> MPKLVTWMNNQRVGELTKLANGAHTFKYAPEWLASRYARPLSLSLPLQRGNITSDAVFNFFDNLLPDSPIVRDRIVKRYHAKSRQPFDLLSEIGRDSVGAVTLIPEDETVTHPIMAWEKLTEARLEEVLTAYKADIPLGMIREENDFRISVAGAQEKTALLRIGNDWCIPKGITPTTHIIKLPIGEIRQPNATLDLSQSVDNEYYCLLLAKELGLNVPDAEIIKAGNVRALAVERFDRRWNARRTVLLRLPQEDMCQTFGLPSSVKYESDGGPGIARIMAFLMGSSEALKDRYDFMKFQVFQWLIGATQGHAKNFSVFIQAGGSYRLTPFYDIISAFPVLGGTGIHISDLKLAMGLNASKGKKTAIDKIYPRHFLATAKVLRFPEVQMHEILS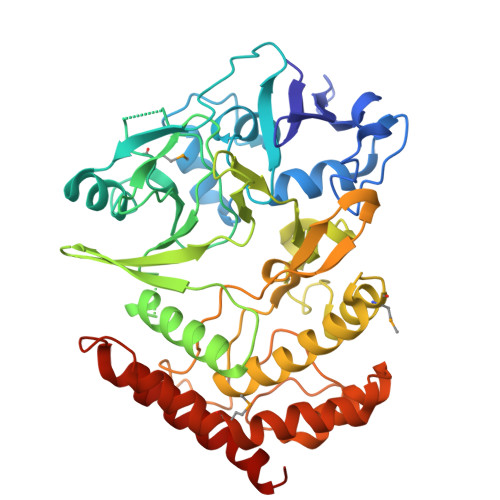DFARMIPAALDNVKTSLPTDFPENVVTAVESNVLRLHGRLSREYGSK>MAHHHHHHADRVHPPAAPPDAQSSGFVFRDEFDGPAGSAPDGSKWVAAKFRERIKNPVFWDRPENMGEYRDSRTNIFLDGNSNLVIRATKEGNKYFSGKLHGTFRGGMGHTFEARIKFNCLTDGCWPA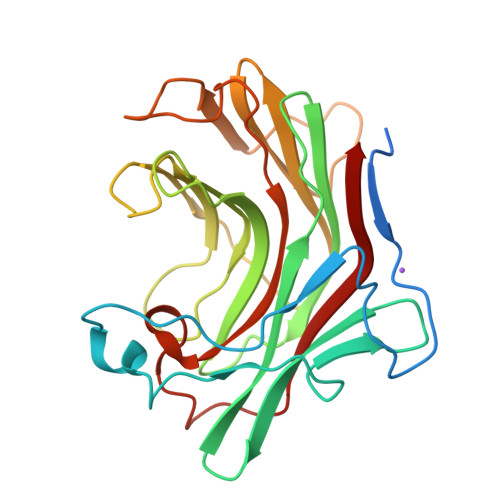WWLLNDNPERGGEIDMAEWYGNRDWPSGTTVHARLDGTSFETLPVPIDSNWHTWRCTWTEAGLYFWMDYHDGMEPYLTVDANSLDDWPFNDPGYTLQPMLNLAVAGSGGGDPAGGSYPAEMLVDYVRVW[2x]> GAPGIAGRIVVLDPGHNGANDSSINNQVPDGRGGTKSCQTSGTATDGGYPEHTFTWNTVLLIRQQLTQLGVRTAMTRGDDNKLGPCIDKRAEIENSYNPDAVVSIHADGGPAGGHGFHVNYSNPPVNAVQGEPTLRFAKTMRDSLQAAGLTPATYIGTGGLYGRSDLAGLNLAQHPKVLVELGNMKNAQDSAMMTSPEGRSKYAQAVVQGIVAYLSGTAPAAAPAPEAAPAGG

PG remodeling is performed by numerous autolysins acting on specific substrates and at different stages during bacterial growth. While glycosidases, such as muraminidases and glucosaminidases act to hydrolyze the glycosidic bonds between the carbohydrate units, peptidases, such as N-acetylmuramyl-l-alanine amidases, l,d-endopeptidases, d,l-endopeptidases, l,d-carboxypeptidases, and dd-carboxypeptidases, hydrolyze the amide bonds of the peptide stem at specific positions. Ami1Mab and Ami1Msm displayed an overall globular structure comprising a central β-sheet (β1, 4, 5, 6, 7, 8) surrounded by strands β2 and β3 forming an antiparallel β-sheet, six α-helices, and one 310 helix (η1). The catalytic zinc is coordinated by the highly-conserved triad which constitutes the amidase_3 motif signature, namely H25, E60, and H115 in Ami1Mab and H51, E86, and H141 in Ami1Msm.

The crystal structure of Ami1Mab was solved at a high resolution in its free form and also bound to l-Ala-d-IsoGln, one of the end-product of the reaction. Ami1Mab was purified without its first 40 amino acids in N-terminus, predicted to correspond to the signal peptide required for secretion. MDP was rapidly hydrolyzed by Ami1Mab, indicating that it is an active PG hydrolase that cleaves the amide bond between the N-acetylmuramic acid and l-Ala. Incubating Ami1Mab with the chelating agent EDTA prior to the reaction almost completely abolished the enzymatic activity. These results demonstrate that, like Ami1Mtb, Zn2+ is required for catalysis of Ami1Mab. To facilitate the search for the potential inhibitor’s binding-site, the Ami1Mab crystal structure was probed with the CASTp server to identify cavities in the protein structure. This analysis led to the identification of a single cavity of a volume of 72 Å2 comprising the active site of Ami1Mab. The three inhibitors could be docked into the Ami1Mab active site with similar binding energy (ΔG°). The proposed docking poses strongly suggest that the three inhibitors are able to occupy the active site in a manner similar to the dipeptide seen in the crystal structure. The docking study supports the view that these inhibitors might act by competing with the binding of the PG peptide stem.>[2x]MAPVGGKKAKKGILERLNAGEIVIGDGGFVFALEKRGYVKAGPWTPEAAVEHPEAVRQ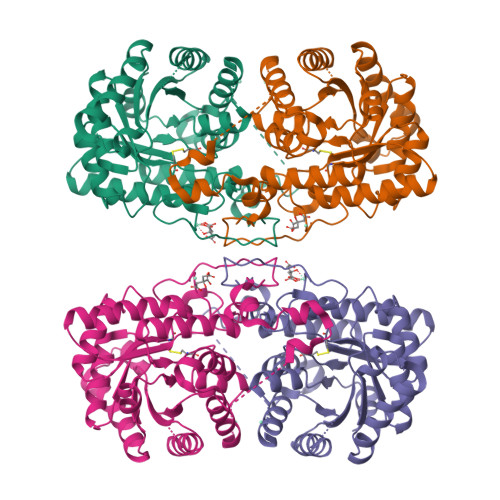LHREFLRAGSNVMQTFTFYASEDKLENRGNYVLEKISGQEVNEAAADIARQVADEGDALVAGGVSQTPSYLSAKSETEVKKVFLQQLEVFMKKNVDFLIAEYFEHVEEAVWAVETLIASGKPVAATMAIGPEGDLHGVPPGEAAVRLVKAGASIIGVNCHFDPTISLKTVKLMKEGLEAAQLKAHLMSQPLAYHTPDANKQGFIDLPEFPFGLEPRVATRWDIQKYAREAYNLGVRYIGGCCGFEPYHIRAIAEELAPERGFLPPASEKHGSWGSGLDMHTKPWVRARARKEYWENLRIASGRPYNPSMSKPDGWGVTKGTAELMQQKEATTEQQLKELFEKQKFKSQ As the first reported host of “non-pathogenic-derived” pili, Lactobacillus rhamnosus GG is a gut-adapted commensal lactic acid bacterium (LAB) and one of many clinically investigated probiotic strains for human use in the prevention and treatment of certain gastric ailments. As with other Gram-positive bacteria, sortase-dependent piliation in L. rhamnosus GG (called SpaCBA) is assembled from the ~30 kDa SpaA (backbone), ~20 kDa SpaB (basal), and ~90 kDa SpaC (tip-located) pilins. Two immunoglobulin (Ig)-like subdomains comprise GG-SpaA, each having the conserved residues of a canonical E-box motif and internal isopeptide bonds formed between either lysine and asparagine or lysine and aspartate residues. Our findings show that the GG-SpaA structure has certain features in common with other pathogen-derived pilin-proteins, such as the Ig-like CnaB-type folds and the presence of internal isopeptide bonds6940.

Prior to obtaining crystals of full-length E269A-substituted GG-SpaA, this mutant protein had fortuitously degraded to only the N-domain during crystallization. Up to now, the crystal structure of an N-terminal domain from a Gram-positive pilin has never been determined before by X-ray crystallography, largely because of its rather flexible nature. Yet, for these particular crystals of the E269A mutant, all N-domain residues were easily built into the electron density map, with the exception of Thr55-Ile57 in the AB loop. Here, the crystal structure of the N-domain exhibited a major conformational change at the domain interface region, but with the overall fold still retained (RMSD of 1 Å). However, isopeptide bonding between Lys47 and Asn172 was no longer visible in the structure. Upon further inspection of the structure, residues (170–180) encompassing the domain linker region exhibit a 34 Å movement towards the AB loop. This structural rearrangement has caused Asn172 to shift 3.5 Å away from its normal WT position, which subsequently prevents isopeptide bond formation. Moreover, the NH group of the Lys47 side chain shows a ∼160° rotation toward Glu139 and forms a salt bridge. The localized perturbations caused by the displacement of the linker region has disrupted its hydrogen-bonding interactions with the neighboring AB and EF loops, thereby moving each of them away (5 and 7 Å, respectively) from the linker residues. From the structure it appears that the C-terminal tail of GG-SpaA (β-strand G) must be properly positioned to create a favorable molecular environment that then facilitates isopeptide bonding in the N-domain.

> MGRDPNSTNDTTTQNVVLTKYGFDKDVTAIDRATDQIWTGDGAKPLQGVDFTIYNVTANYWASPKDYKGSFDSAPVAATGTTNDKGQLTQALPIQSKDASGKTRAAVYLFHETNPRAGYNTSADFWLTLPAKAAADGNVYVYPKNVQKTTYER LysR-type transcriptional regulators (LTTRs), which constitute one of the largest protein families in prokaryotes, regulate transcription by sensing specific effector molecules. Two conserved domains in LTTRs, the N-terminal DNA binding domain (DBD) and the C-terminal effector binding domain (EBD) are connected by a single linker helix (LH). YhaJ, which is an LTTR family member, has been exploited for the detection of explosives such as soil-buried landmines. The YhaJ transcription factor responds to dinitrophenol (DNT) and its metabolic products.

The YhaJ DNA binding domain linked to a linker region (named YhaJ-DBD, residues 1-93) with a C-terminus hexahistidine tag was purified using affinity chromatography and size exclusion chromatography. The crystal structure of YhaJ-DBD was determined at 1.76 Å resolution and refined to R-work and R-free values of 17.3 and 21.8%, respectively. The asymmetric unit contained a dimer of YhaJ-DBD’s. The YhaJ-DBD structure adopts a winged-helix-turn-helix fold typically seen in LTTR family proteins. Three α-helices (α1 [Leu9-Arg21], α2 [Phe24-Gly32], and α3 [Pro35-Asp50]) constitute the DNA binding region, followed by a winged region (WR) (Val51-Thr64) and a long linker helix (LH) (α4 [Asn65-Arg93]). Hydrophobic residues in the α1 - α3 helices (α1 [Ala11, Leu12, Val14, Met15, and Ile18], α2 [Phe24, Ala27, and Leu31], and α3 [Met42, Leu45, and Leu49]) form a strong hydrophobic core of the DBD. Residues in the LH of one monomer interact with those of the other monomer mainly by hydrophobic interactions. In the dimer, two charged residues Arg73 and Asp87 in one LH interact with Asp87 and Arg73 of the other LH, respectively, stabilizing an anti-parallel orientation of LH’s. In the YhaJ-DBD:DNA complex model, YhaJ-DBD interacts with the major groove of the target DNA. Positive residues (Arg33, Lys44, Arg56, and Arg60) of YhaJ-DBD interact with negative-charged phosphate groups in nucleotides.

>[2x]MAKERALTLEALRVMDAIDRRGSFAAAADELGRVPSALSYTMQKLEEELDVVLFDRSGHRTKFTNVGRMLLERGRVLLEAADKLTTDAEALARLEHHHHHH N-[(1S)-1-{1-[(1R,3E)-1-ACETYLPENT-3-EN-1-YL]-1H-1,2,3-TRIAZOL-4-YL}-1,2-DIMETHYLPROPYL]BENZAMIDE 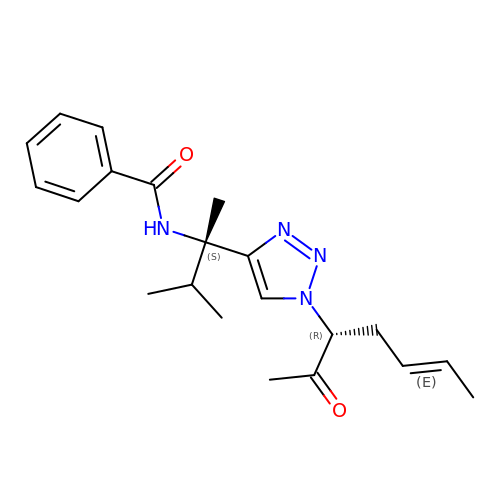| C21 H28 N4 O2 | OEHUTYXPQSSKAK-RVLLMHTFSA-N> MNSEELERESEEAERRLQEARKRSEEARERGDLKELAEALIEEARAVQELARVACERGNSEEAERASEKAQRVLEEARKVSEEAREQGDDEVLALALIAIALAVLALAEVACCRGNSEEAERASEKAQRVLEEARKVSEEAREQGDDEVLALALIAIALAVLALAEVACCRGNKEEAERAYEDARRVEEEARKVKESAEEQGDSEVKRLAEEAEQLAREARRHVQECRGGW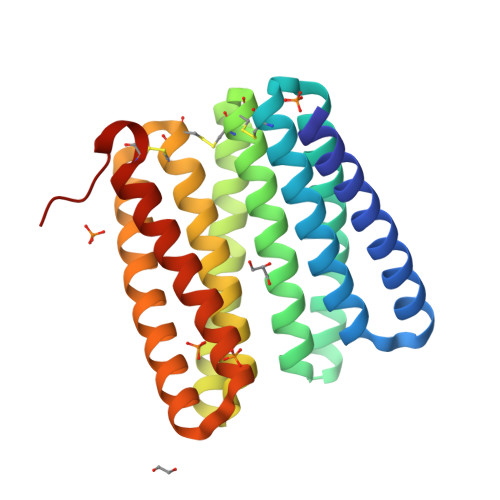LEHHHHHH> SANEDMPVEKILEAELAVEPKTETYVEANMGLNPSSPNDPVTNICQAADKQLFTLVEWAKRIPHFSELPLDDQVILLRAGWNELLIASFSHRSIAVKDGILLATGLHVHRNSAHSAGVGAIFDRVLTELVSKMRDMQMDKTELGCLRAIVLFNPDSKGLSNPAEVEALREKVYASLEAYCKHKYPEQPGRFAKLLLRLPALRSIGLKCLEHLFFFKLIGDTPIDTFLMEMLEA;> PEVGELIEKVRKAHQETFPALCQLGKYTTNNSSEQRVSL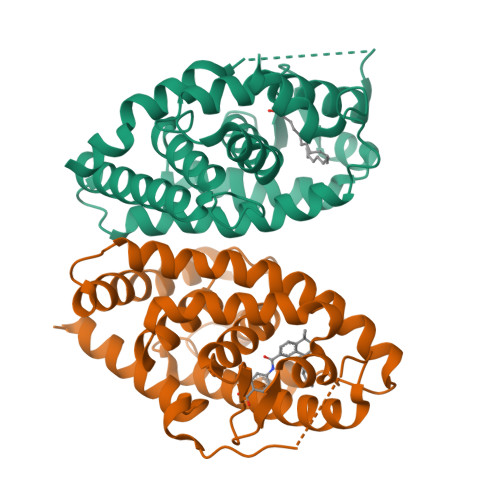DIDLWDKFSELSTKCIIKTVEFAKQLPGFTTLTIADQITLLKAACLDILILRICTRYTPEQDTMTFSDGLTLNRTQMHNAGFGPLTDLVFAFANQLLPLEMDDAETGLLSAICLICGDRQDLEQPDRVDMLQEPLLEALKVYVRKRRPSRPHMFPKMLMKITDLRSISAKGAERVITLKMEIPGSMPPLIQEMLEN> MKDRFELVSKYQPQGDQPKAIEKLVKGIQEGKKHQTLLGATGTGKTFTVSNLIKEVNKPTLVIAHNKTLAGQLYSEFKEFFPNNAVEYFVSYYDYYQPEAYVPQTDTFIEKDASINDEIDKLRHSATSALFERRDVIIIASVSCIYGLGSPEEYREMVVSLRTEMEIERNELLRKLVDIQYARNDIDFQRGTFRVRGDVVEIFPASRDEHCVRVEFFGDEIERIREVDALTGEILGDRDHVAIFPASHFVTRAEKMEKAIQNIEKELEEQLKVMHENGKLLEAQRLEQRTRYDLEMMREMGFCSGIENYSRHLTLRPPGSTPYTLLDYFPDDFMIVVDESHVTIPQVRGMFNGDQARKQVLVDHGFRLPSALDNRPLRFEEFEKHMHNIVYVSATPGPYEIEHTDEMVEQIIRPTGLLDPLIDVRPIEGQIDDLIGEIQARIERNERVLVTTLTKKMSEDLTDYLKEIGIKVNYLHSEIKTLERIEIIRDLRLGKYDVLVGINLLREGLDIPEV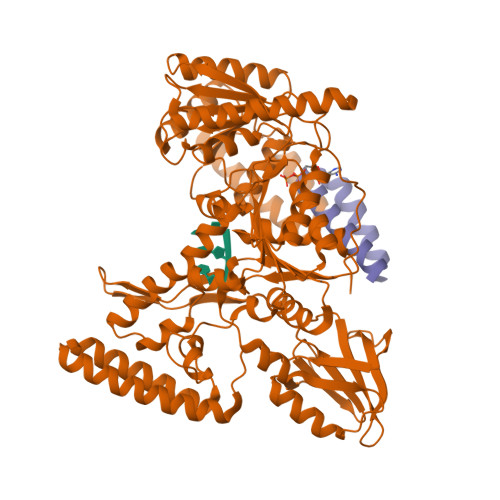SLVAILDADKEGFLRSERSLIQTIGRAARNAEGRVIMYADKITKSMEIAINETKRRREQQERFNEEHGITPKTINKEIRDVIRATVAAEDKAEYKTKAAPKLSKMTKKERQKVVEQMEHEMKEAAKALDFERAAELRDLLLELKAEG;> KERQKVVEQMEHEMKEAAKALDFERAAELRDLLLELKAEG Among these, group 21 allergens including Blo t 217, Der p 218 and Der f 219 identified in B. tropicalis, D. pteronyssinus and D. farinae, respectively, are known as mid-tier allergens in the allergic response. The structure of rDer f 21 adopts a bundle of three anti-parallel α-helices similar to the group 21 HDM allergen Blo t 2116, and group 5 HDM allergens including Blo t 514,15 and Der p 512. The crystal structure of rDer f 21 revealed an elongated dimer structure with molecules A and B interacting in a head-to-toe orientation. Helices α1 and α2 form an intermolecular anti-parallel dimeric interface while the C-terminal α-helix (α3) is fully exposed to the solvent.

The structures of rDer f 21 were obtained from two different crystal forms grown using either PEG 400 or PEG 2000 MME as a precipitant. The similar dimeric form of rDer f 21 protein crystal structure grown from the solution containing PEG 2000 MME, rDer f 21PEG2KMME, was solved to 2.3 Å resolution. This crystal contains four molecules per asymmetric unit, which represent two dimers of rDer f 21. Although the rDer f 21 protein structure crystallized with PEG 2K MME as a precipitant neither shows the helical distortion nor binds a molecule of PEG 2K MME, some unidentified weak electron density was also observed in the cavity. Furthermore, knowing that only PEG 400 but not PEG 2K MME can fit within the cavity, we further deduce that a molecule of a size similar to PEG400 may exist as a physiologically active molecule for Der f 21.

>MHHHHHHSSGLVPRGSEDKWRNAFDHMLMEEFEEKMDQIEHGLLMLSEQYKELEKTKSKELKEQILRELTIAENYLRGALKFMQQEAKRTDLNMFERYNFETAVSTIEILVKDLAELAKKVKAVKSDD[4x]>[2x]MLSFLLTLKRMLRACLRAWKDKEFQVLFVLTILTLISGTIFYSTVEGLRPI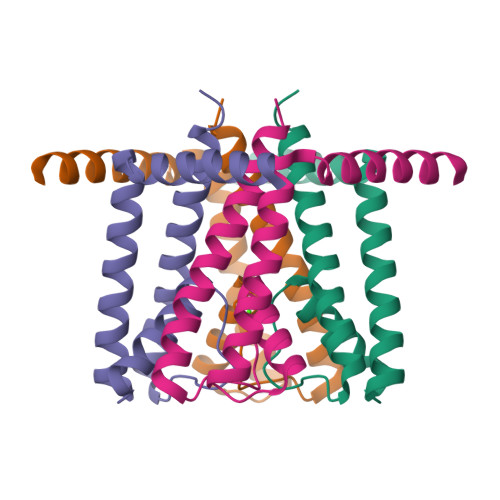DALYFSVVTLTTVGNGNFSPQTDFGKIFTILYIFIGIGLVFGFIHKLAVNVQLPSILSNLVPR> MGRIKNKQFAVIGLGRF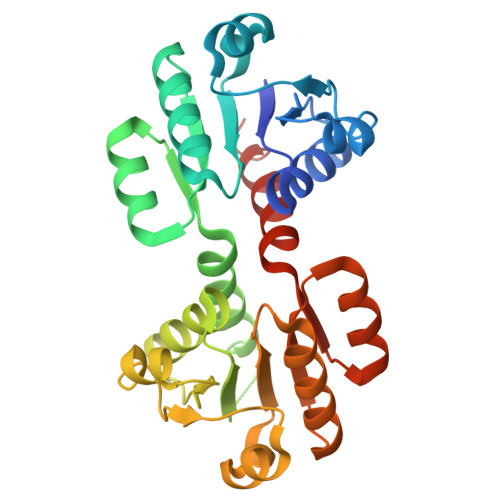GGSIVKELHRMGHEVLAVDINEEKVNAYASYATHAVIANATEENELLSLGIRNFEYVIVAIGANIQASTLTTLLLKELDIPNIWVKAQNYYHHKVLEKIGADRIIHPEKDMGVKIAQSLSDENVLNYLEGSKQFAVIGLGRFGGSIVKELHRMGHEVLAVDINEEKVNAYASYATHAVIANATEENELLSLGIRNFEYVIVAIGANIQASTLTTLLLKELDIPNIWVKAQNYYHHKVLEKIGADRIIHPEKDMGVKIAQSLSDENLELVPR> SNAMSLILDDIILSLTNANERTPPQALKTTLSLLYEKSKQYGLSSPQLQALVRLLCETSIIDTVTKVYIVENCFLPDGYLTKELLLEIINHLGTPTVFSRYRIQTPPVLQSALCKWLVHVYFLFPVHSEREHNISSSIWLHLWQFSFLQKWITPLVIWQATTPVDVKPWKLSIIKRCAMHPGYRDAPGSATLILQRFQCLVGASSQITESIITINCNRKTLKSHRNLKLDAHFLSILKRILSRAHPANFPADTVQNTIDMYLSEIHQLGADSIYPLRLQSLPEYVPSDSTVSLWDVTSLEQLAQNWPQLHIPNDVDYMMKPSLNSNVLLPRKVMSRDSLKHLYSSIILIKNSRDESSSPYEWCIWQLKRCFAHQIETPQEVIPIIISVSSMDNKLSSRIIQTFCNLKYLKLDELTLKKVCGGILPLWKPELISGTREFFVKFMASIFMWSTRDGHDNNCTFSETCFYVLQMITNWVLDDKLIALGLTLLHDMQSLLTLDKIFNNATSNRFSTMAFISSLDILTQLSKQTKSDYAIQYLIVGPDIMNKVFSSDDPLLLSAACRYLVATKNKLMQYPSTNKFVRMQNQYIMDLTNYLYRNKVLSSKSLFGVSPDFFKQILENLYIPTADFKNAKFFTITGIPALSYICIIILRRLETAENTKIKFTSGIINEETFNNFFRVHHDEIGQHGWIKGVNNIHDLRVKILM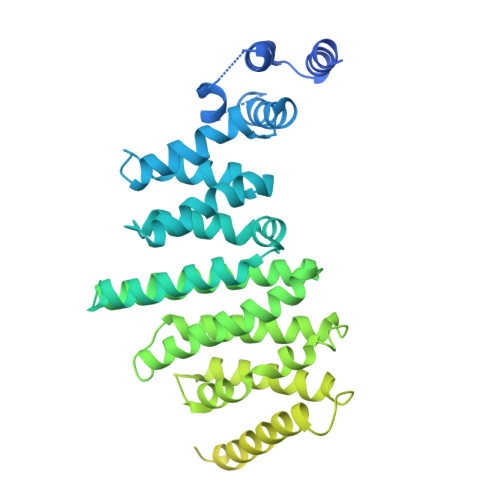HLSNTANPYRDIAAFLFTYLKSLSKYSVQNSXXXXXXXXXXXXXXXXXXXXXXXXXXXXXXXXXXXXX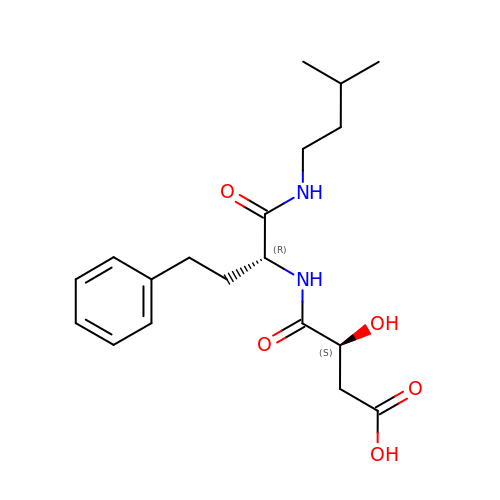N-[3-CARBOXY-2-HYDROXY-PROPIONYL]-D-HOMOPHENYLALANYL-AMINO-2-METHYLBUTANE | C19 H28 N2 O5 | KVZMXOVSHIMGNA-CVEARBPZSA-N5-oxidanyl-1~{H}-pyrimidine-2,4-dione | C4 H4 N2 O3 | 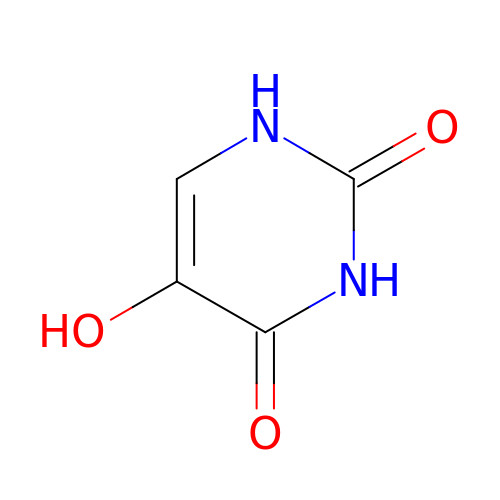OFJNVANOCZHTMW-UHFFFAOYSA-N(3R)-3-amino-2,2-difluoro-3-(4-methoxyphenyl)propanoic acid 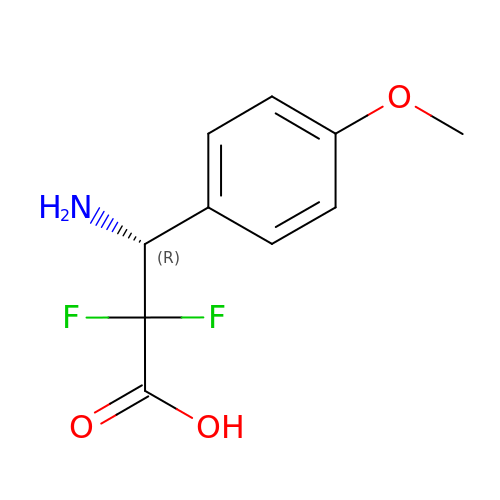| C10 H11 F2 N O3 | LSCGPDBHPYAPAB-MRVPVSSYSA-N>MKPSPEILALRWKDTSAHYSPHEWVAARNVVTANKAALADYFYESMLADPNAAFFLSDQLVKTKLHASMQDWLESVYAAAPTEEYERTVAFQRKVGEVHARIDIPVHLVTRGASALIRRICELLDRDASLSAAQAAATCRYVADVTMTAVEMMSHAYSVSHDRNARAEELE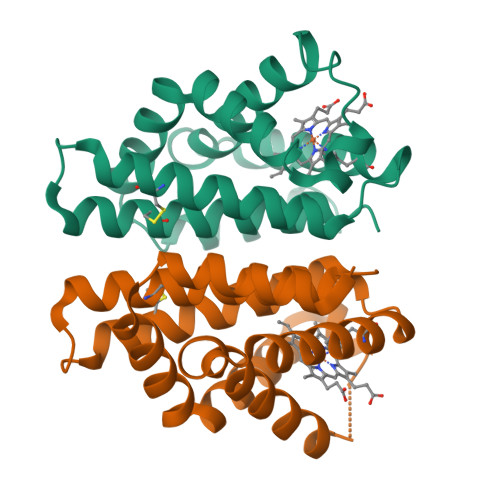HHHHHH[2x]> 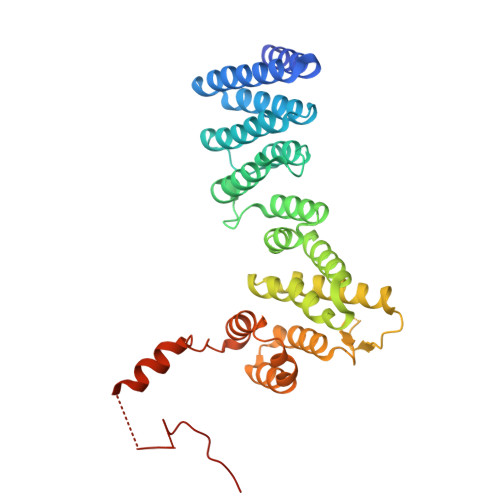MGHHHHHHSNKIERIIARLQRRIAEGQPEEQYEAAQETRLVAARYSKQGNWAAAVDILASVSQTLLRSGQGGSGGDLAVLLVDTFRQAGQRVDGASRGKLLGCLRLFQPGEPVRKRFVKEMIDWSKKFGDYPAGDPELHHVVGTLYVEEGEFEAAEKHLVLGTKESPEVLARMEYEWYKQDESHTAPLYCARAVLPYLLVANVRAANTAYRIFTSALVEDNKGLTVQNIGSQSAELRIFPSLPLLNFISMLLLSVQKGSPDLFRQLKSKYEANLNELNGIWDTALELIAEMYFGIQRPRQSNPLLDMMGSLFGGGGGAPSKAALRRIDTPAAEGLD> MHHHHHHHDGTENPIHDRTSDYHKYLKVKQGDSDLFKLTVSDKRYIWYNPDPKERDSYECGEIVSETSDSFTFKTVDGQDRQVKKDDANQRNPIKFDGVEDMSELSYLNEPAVFHNLRVRYNQDLIYTYSGLFLVAVNPFKRIPIYTQEMVDIFKGRRRNEVAPHIFAISDVAYRSMLDDRQNQSLLITGESGAGKTENTKKVIQYLASVAGRNQANGSGVLEQQILQANPILEAFGNAKTTRNNNSSRFGKFIEIQFNSAGFISGASIQSYLLEKSRVVFQSETERNYHIFYQLLAGATAEEKKALHLAGPESFNYLNQSGCVDIKGVSDSEEFKITRQAMDIVGFSQEEQMSIFKIIAGILHLGNIKFEKGAGEGAVLKDKTALNAASTVFGVNPSVLEKALMEPRILAGRDLVAQHLNVEKSSSSRDALVKALYGRLFLWLVKKINNVLCQERKAYFIGVLDISGFEIFKVNSFEQLCINYTNEKLQQFFNHHMFKLEQEEYLKEKINWTFIDFGLDSQATIDLIDGRQPPGILALLDEQSVFPNATDNTLITKLHSHFSKKNAKYEEPRFSKTEFGVTHYAGQV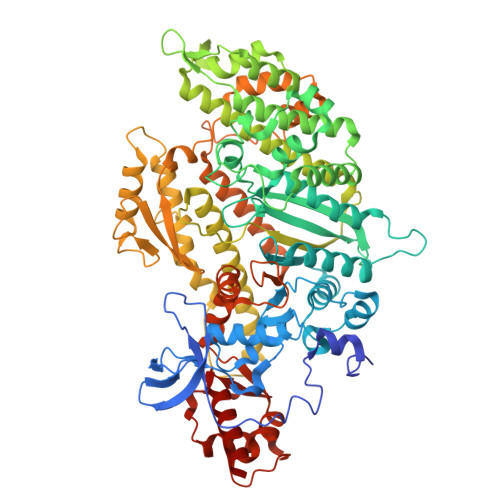MYEIQDWLEKNKDPLQQDLELCFKDSSDNVVTKLFNDPNIASRAKKGANFITVAAQYKEQLASLMATLETTNPHFVRCIIPNNKQLPAKLEDKVVLDQLRCNGVLEGIRITRKGFPNRIIYADFVKRYYLLAPNVPRDAEDSQKATDAVLKHLNIDPEQYRFGITKIFFRAGQLARIEEAREQRISEI>GPAGAQDDVPPYFKTEPVRTQVRLEGSRLVLTCMAEGSWPLEFKWLHNNRELTRFSLEYRYMITSLDRTHAGFYRCIVRNRMGALLQRQTEVQVAYMGSFEEGEKRQSVNHGEAAVIRAPRISSFPRPQVTWFRDGRKIPPSSRIAITLENTLVILSTVAPDAGRYYVQAVNDKNGDNKTSQPITLAVENVGGPADPIAPTIIIPPKNTSVVAGTSEVTMECVANARPLIKLHIVWKKDGAPLSSGISDYNRRLTIANPTVSDAGYYECEAMLRSSSVAPVTRGAYLSVLEPPQFVREPERHITAEMEKVVDIPCRAKGVPP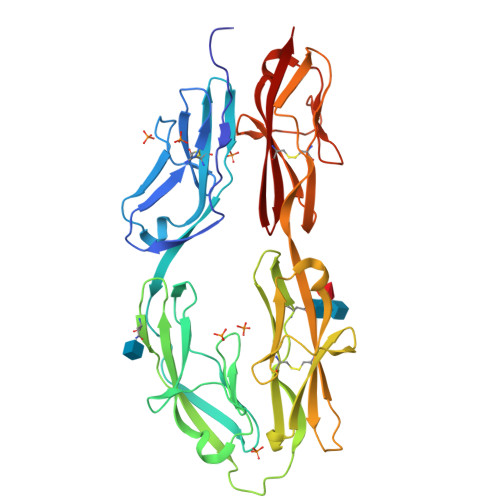PSITWYKDAALVEVGKLTRFKQRSDGGLQISGLLPDDTGMLQCFAHNAAGEAQTSTYLAVTS[4x]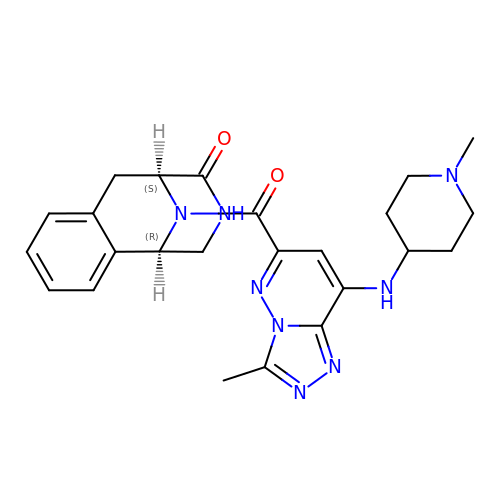(1R,9S)-13-[[3-methyl-8-[(1-methylpiperidin-4-yl)amino]-[1,2,4]triazolo[4,3-b]pyridazin-6-yl]carbonyl]-11,13-diazatricyclo[7.3.1.0^{2,7}]trideca-2,4,6-trien-10-one | C24 H28 N8 O2 | JFALEKLXZVKEKY-SFTDATJTSA-N> MFSAGHKIKGTVVLMPKNELEVNPDGSAVDNLNAFLGRSVSLQLISATKADAHGKGKVGKDTFLEGINTSLPTLGAGESAFNIHFEWDGSMGIPGAFYIKNYMQVEFFLKSLTLEAISNQGTIRFVCNSWVYNTKLYKSVRIFFANHTYVPSETPAPLVSYREEELKSLRGNGTGERKEYDRIYDYDVYNDLGNPDKSEKLARPVLGGSSTFPYPRRGRTGRGPTVTDPNTEKQGEVFYVPRDENLGHLKSKDALEIGTKSLSQIVQPAFESAFDLKSTPIEFHSFQDVHDLYEGGIKLPRDVISTIIPLPVIKELYRTDGQHILKFPQPHVVQVSQSAWMTDEEFAREMIAGVNPCVIRGLEEFPPKSNLDPAIYGDQSSKITADSLDLDGYTMDEALGSRRLFMLDYHDIFMPYVRQINQLNSAKTYATRTILFLREDGTLKPVAIELSLPHSAGDLSAAVSQVVLPAKEGVESTIWLLAKAYVIVNDSCYHQLMSHWLNTHAAMEPFVIATHRHLSVLHPIYKLLTPHYRNNMNINALARQSLINANGIIETTFLPSKYSVEMSSAVYKNWVFTDQALPADLIKRGVAIKDPSTPHGVRLLIEDYPYAADGLEIWAAIKTWVQEYVPLYYARDDDVKNDSELQHWWKEAVEKGHGDLKDKPWWPKLQTLEDLVEVCLIIIWIASALHAAVNFGEYPYGGLI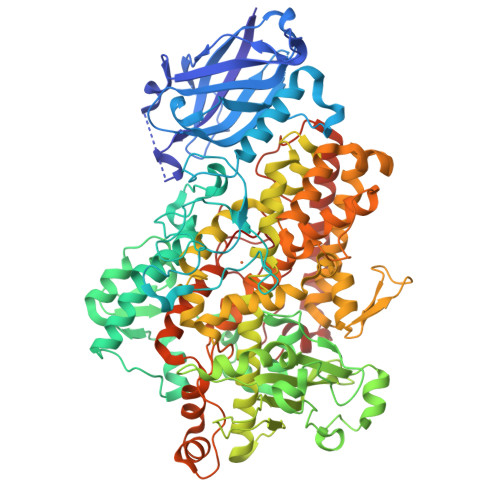MNRPTASRRLLPEKGTPEYEEMINNHEKAYLRTITSKLPTLISLSVIEILSTHASDEVYLGQRDNPHWTSDSKALQAFQKFGNKLKEIEEKLVRRNNDPSLQGNRLGPVQLPYTLLYPSSEEGLTFRGIPNSISI> ANRTLIVTTILEEPYVMYRKSDKPLYGNDRFEGYCLDLLKELSNILGFIYDVKLVPDGKYGAQNDKGEWNGMVKELIDHRADLAVAPLTITYVREKV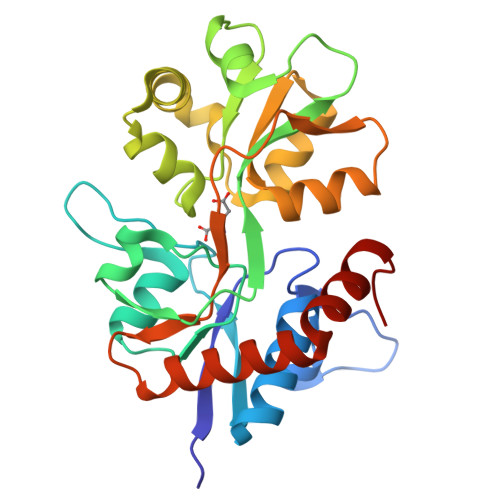IDFSKPFMTLGISILYRKGTPIDSADDLAKQTKIEYGAVRDGSTMTFFKKSKISTYEKMWAFMSSRQQTALVRNSDEGIQRVLTTDYALLMESTSIEYVTQRNCNLTQIGGLIDSKGYGVGTPIGSPYRDKITIAILQLQEEGKLHMMKEKWWRGNGCP>[2x]MQTSLFEFANVLITAVKEASYSISKFKEEVEIKYKSDGSEVTQVDTQSQQIIFSIIKNKYPTINIIGEEDVENGIPDNQLPTITQLSFGSLENKIININDIIIYVDPLDGTDC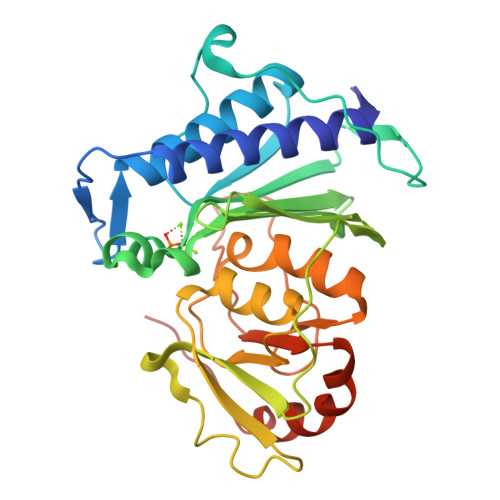YTHKQYDSVCVLVGVTYKGKPMIGIVSKPFYNNEITFAIENYISSISLQPLNDKIIFVCSKKNDIQHLIKSFPDPYEVKYKGGSGAKMMAIIHQEADIYYHPLIQSCTWDTLAAQVILEAQGGIVCDIYGNPLCYPSSKKESMRHKKGVLCLSPRAKKYLPYMLSISKTILLLQHHHHHH>[3x]QDADKLPHTKVTLVAPPQVHPHEQATKSGPKVVEFTMTIEEKKMVIDDKGTTLQAMTFNGSMPGPTLVVHEGDYVQLTLVNPATNAMPHNVDFHGATGALGGAKLTNVNPGEQAT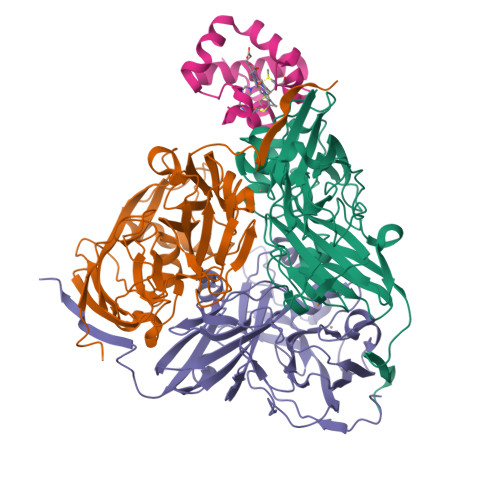LRFKADRSGTFVYHCAPEGMVPWHVVSGMSGTLMVLPRDGLKDPQGKPLHYDRAYTIGEFDLYIPKGPDGKYKDYATLAESYGDTVQVMRTLTPSHIVFNGKVGALTGANALTAKVGETVLLIHSQANRDTRPHLIGGHGDWVWETGKFANPPQRDLETWFIRGGSAGAALYTFKQPGVYAYLNHNLIEAFELGAAGHIKVEGKWNDDLMKQIKAPAPIPR;> AADAPAQLDPAGEKLYRSACVVCHASGVANAPKLGDKQAWAPFLAQGADALLATVLKGKGAMPPRGGTAADEATLRAAVAYMMDAAR> DMPERFDAFICYCPSDIQFVQEMIRQLEQTNYRLKLCVSDRDVLPGTCVWSIASELIEKRCRRMVVVVSDDYLQSKECDFQTKFALSLSPGAHQKRLIPIKYKAMKKEFPSILRFITVCDYTNPCTKSWFWTRLAKAL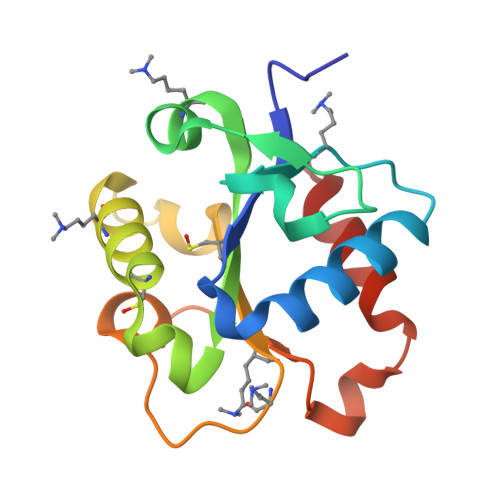SLP2-[6-(1-hydroxycyclohexyl)pyridin-2-yl]-1H-indole-5-carboximidamide | C20 H22 N4 O | 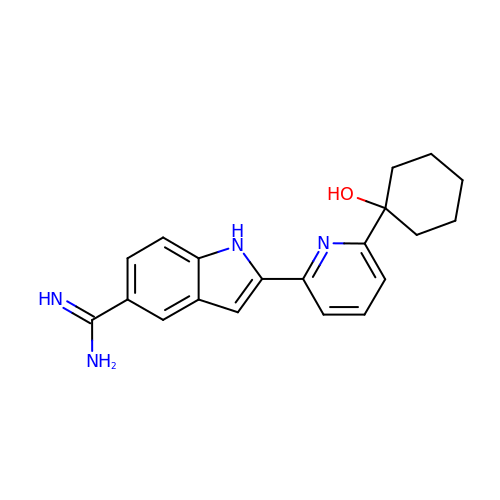VXVYXKAPTSJLCT-UHFFFAOYSA-N>SVGTFSLPALPYAYDALEPSISAQIMELHHSKHHQTYVTNLNNALKTYSTALAANDVPSQIALQAAIKFNGGQHINHSLFWENLCPASSPDADPASAPELTAEIAKTWGSLDKFKEAMGKALLGIQGSGWGWLVKEGSGLRIVTTKDGDPVVGGEVPVFGIDMWEHAYYLQYLNGKAAYVDNIWKVINWKTAEQRFKGDREDAF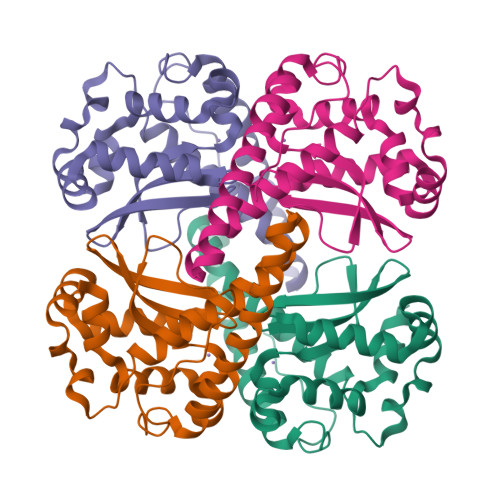KILKASL[4x]> HHHHHHMAKKVNWYVSSSPRSPEKIQPELKVLANFEGSYWKGVKGYKAQEAFAKELAALPQFLGTTYKKEAAFSTRDRVAPMKTYGFVFVDEEGYLRITEAGKMLANNRRPKDVFLKQLVKWQYPSFQHKGKEYPEEEWSINPLVFVLSLLKKVGGLSKLDIAMFSLTATNNNQVDEIAEEIMQFRNEREKIKGQNKKLEFTENYFFKRFEKIYGNVGKIREGKSDSSHKSKIETKMRNARDVADATTRYFRYTGLFVARGNQLVLNPEKSDLIDEIISSSKVVKNYTRVEEFHEYYGNPSLPQFSFETKEQLLDLAHRIRDENTRLAEQLVEHFPNVKVEIQVLEDIYNSLNKKVDVETLKDVIYHAKELQLELKKKKLQADFNDPRQLEEVIDLLEVYHEKKNVIEEKIKARFIANKNTVFEWLTWNGFIILGNALEYKNNFVIDEE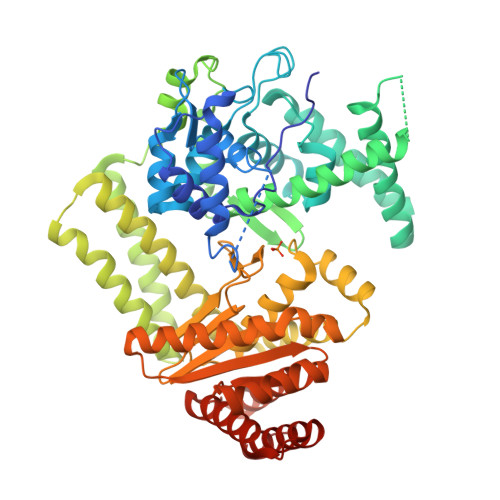LQPVTHAAGNQPDMEIIYEDFIVLGEVTTSKGATQFKMESEPVTRHYLNKKKELEKQGVEKELYSLFIAPEINKNTFEEFMKYNIVQNTRIIPLSLKQFNMLLMVQKKLIEKGRRLSSYDIKNLMVSLYRTTIESERKYTQIKAGLEETLNNWVVDKEVRF SK catalyzes the specific phosphorylation of the 3-hydroxyl group of shikimic acid, using ATP as a co-substrate. The shikimate pathway is comprised of seven enzymatic components that convert erythrose 4-phosphate and phosphoenolpyruvate into chorismate, for subsequent synthesis of aromatic compounds. SKs belong to a class of P-loop kinases that share a homologous α-β-α fold. Overall, these structures have a characteristic α-β-α fold that consists of the CORE domain (residues 1–31, 61–108, and 124–162), the SB domain (residues 32–60), and the LID region (residues 109–123) in the monomer.

We also determined the X-ray structure of the E114A mutant SK-inhibitor complex using a selective inhibitor (NSC162535; IC50 = 4.9 µM) identified from virtual docking analysis. After extensive trials, only the map of the E114A·162535 crystal showed a large piece of residual density in the binding pocket, which could be modeled as NSC162535. The final E114A·162535 crystal structure shows a trimeric assembly (R = 21.8%, Rfree = 26.2%). NSC162535, which is clearly observed in two of the three subunits, exhibits an extended conformation between LID and SB. Interestingly, it extends out to the entrance of the binding pocket. The LID loop of HpSK accommodates the inhibitor by undergoing a large conformational switch, distinct from that of HpSK·SO4 and HpSK• S3P•ADP. Notably, the side chain of R116 at LID forms hydrogen bonds with an SO4 group and packs against one of the naphthalene moieties with an electron-rich π system. This naphthalene group also packs against the aromatic ring of F48 from the SB domain on the other side, establishing strong cation-π and π-π interactions. The other naphthalene group interacts with the side chain of R132, yielding a cation-π interaction. Additionally, the guanidino groups of R116 and R57 are located near the diazo moiety of NSC162535, making cation-π interaction and a kind of polar interaction, respectively.

>MQHLVLIGFMGSGKSSLAQELGLALKLEVLDTDMIISERVGLSVREIFEELGEDNFRMFEKNLIDELKTLKTPHVISTGGGIVMHENLKGLGTTFYLKMDFETLIKRLNQKERAKRPLLNNLTQAKELFEKRQALYEKNASFIIDARGGLNNSLKQVLQFIALQPSLS[3x]> MYLTKEEELILAGEYGYALQKAMEILVALGDIYGADRLIPIKSAQV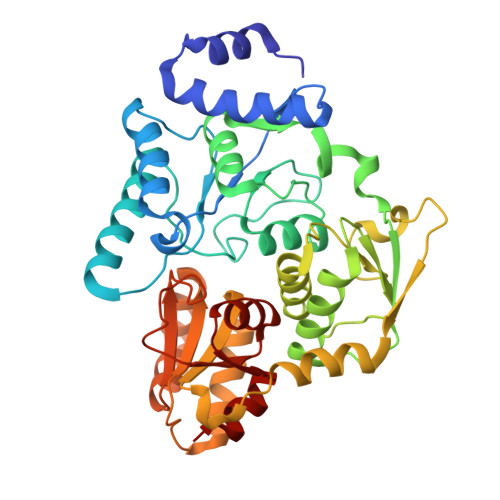AGVSYKNIGDAGIEFLRDFVEAGAKVSVYTTLNPAGIGDDEFMEKQMEVLELYRKMGIEVTSTCTPYYGANLPKFGDHIAWSESSAVSFANSILGARTNREGGPSSLAAAIVGKTPNYGLHLDENRKATVIVDVKAKVKTFADYSVLGYHVGKTLGNDVPYFKNLKPEKTEFLKELGAAMGATGSIALYHVEGETPEYREAITDKLETITVEDSDLKAVRESFQDDWSDIDMILIGCPHASLPEVKEIAELLRMRGKPLKIPLFITASRAVKALADALGYTEIIERYNGKIIPDSCFVVSPIKGWYRGIATNSGKSAFYFRSFGFSVRLDDVENLIKEAP> MSGNREQVFPTRMTLGLMKTKLKGANQGYSLLKRKSEALTKRFRDITKRIDDAKQKMGRVMQTAAFSLAEVSYATGENIGYQ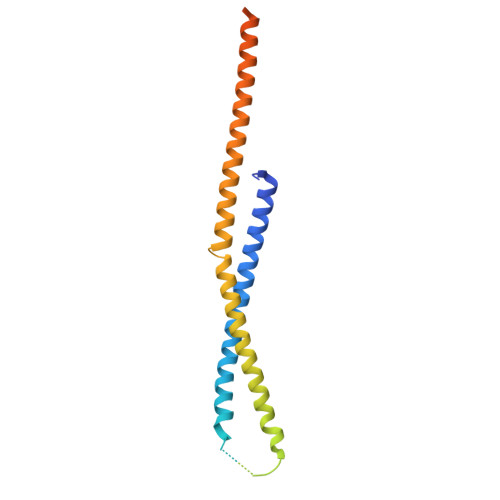VQESVSTARFKVRARQENVSGVYLSQFESYIDPEINDFRLTGLGRGGQQVQRAKEIYSRAVETLVELASLQTAFIILDEVIKVTNRRVNAIEHVIIPRTENTIAYINSELDELDREEFYRLKKVQEKKQNETAKLDAEMKLKRDRAEQDASEVAADEEPQGETLVADQEDDVIF>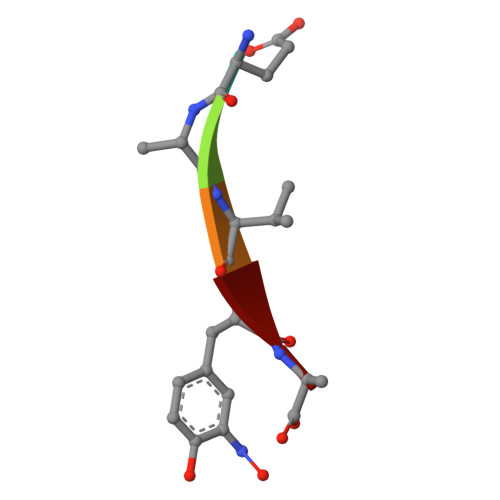 EAVYA>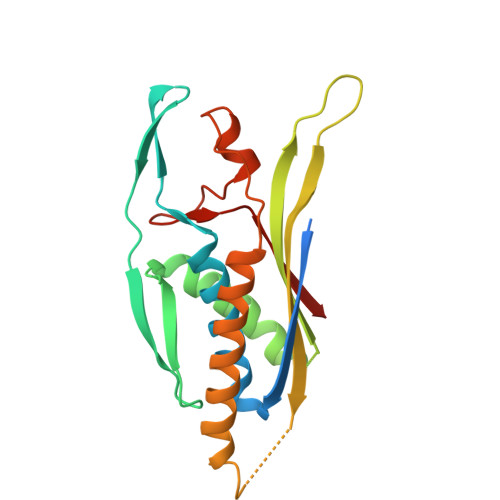 GGTSEDELPPQVHKVGSDEAMNCRSEVLEVSVEGRQVEEAMLAVLHTVLLHRSTGKFHYKKEGTYSIGTVGTQDVDCDFIDFTYVRVSSEELDRALRKVVGEFKDALRNSGGDGLGQMSLEFYQKKKSRWPFSDECIPWEVWTVKVHVVALATEQERQICREKVGEKLCEKIINIVEVMNRHEYLPKMPTQSEVDNVFDTGLRDVQPYLYKISFQITD coproporphyrin 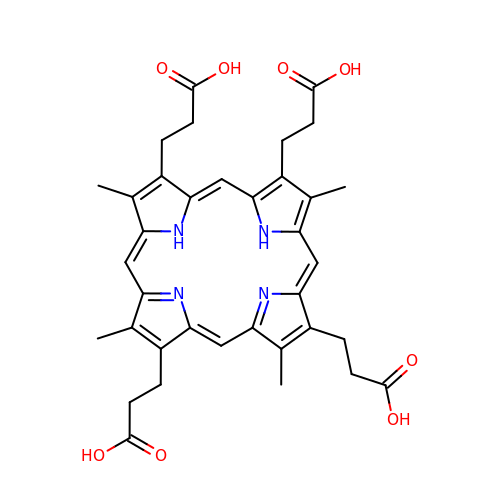III | C36 H38 N4 O8 | XNBNKCLBGTWWSD-UJJXFSCMSA-N>[2x]MSSSKQYQQQPEDEELGPVTIAEDEVEEILDVEDPDGDVAMGSDDEGPEEIALENDSIAYFDGHKDSVFAIAQHPLYPNIVATGGSEGDADDAPGKGYVLDISAAAGRPVLPPSYNSDPSSAPQQNTSLNPIFEIDGHTDSINALTFTLPRGDFLVSGGMDGRMRVYAVSVPQNGALAQFKFLAESQETEEINWFAPCPSPDHPNTIALGASDGSVWVFTLDASDPSNPVQIVQSYFLHTGPCTAGAW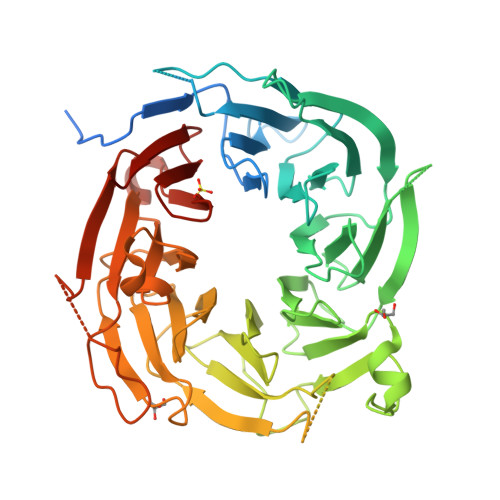SPDGLLLATVSEDESLHVYDVFGVAASKSLVTDNGQTVVSLTNVDQRFAVEGGLFSVAVSPTGAVVAVGGAGGQIKIVGLPRLSQPQQPQSQSQSRTGKAPAGRAGRPSQQQQTTSHQAGTILASLQIQSDNIESLAFSPSAPILAAGSTDGSIAVFDTSRSFALRRHLRGAHAEDPVVKVEFVKSPPNAAMAGWLLTSCGMDGVVRRWDLRGGTAGPGTLPHMQHLQQQRQQQQEGAAPSGLVKEWKGHRSGQEGGGVLGFVQGETGERIVTVGDDAVVLVFEAGSHHHHHH>[2x]KAFAKFPSSASISP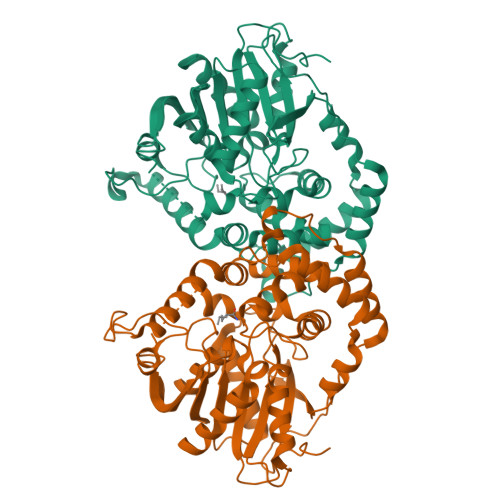NPFTVSIPDEQLDDLKTLVRLSKIAPPTYESLQADGRFGITSEWLTTMREKWLSEFDWRPFEARLNSFPQFTTEIEGLTIHFAALFSEREDAVPIALLHGWPGSFVEFYPILQLFREEYTPETLPFHLVVPSLPGYTFSSGPPLDKDFGLMDNARVVDQLMKDLGFGSGYIIQGGDIGSFVGRLLGVGFDACKAVHLNLCAMRAPPEGPSIESLSAAEKEGIARMEKFMTDGLAYAMEHSTRPSTIGHVLSSSPIALLAWIGEKYLQWVDKPLPSETILEMVSLYWLTESFPRAIHTYRETTPTASAPNGATMLQKELYIHKPFGFSFFPKDLCPVPRSWIATTGNLVFFRDHAEGGHFAALERPRELKTDLTAFVEQVW> MIMDKSIPKATAKRLSLYYRIFKRFNTDGIEKASSKQIADALGIDSATVRRDFSYFGELGRRGFGYDVKKLMNFFAEILNDHSTTNVMLVGCGNIGRALLHYRFHDRNKMQISMAFDLDSNDLVGKTTEDGIPVYGISTINDHLIDSDIETAILTVPSTEAQEVADILVKAGIKGILSFSPVHLTLPKDIIVQYVDLTSELQTLLYFMNQQR

In many Gram-positive bacteria, the redox-sensing transcriptional repressor Rex controls central carbon and energy metabolism by sensing the intra cellular balance between the reduced and oxidized forms of nicotinamide adenine dinucleotide; the NADH/NAD+ ratio. Here, we report high-resolution crystal structures and characterization of a Rex ortholog (Gbs1167) in the opportunistic pathogen, Streptococcus agalactiae, also known as group B streptococcus (GBS). Rex is a homodimer consisting of two domains, an N-terminal DNA recognition domain and a C-terminal Rossmann-like dinucleotide-binding and dimerization domain. The dimerization of Rex is stabilized by the swapping of the C-terminal α-helices and the dimer binds to a consensus Rex OPerator (ROP) sequence (TTGTGAAN4TTCACAA) to repress expression of target genes.

The structure of Rex in complex with a palindromic 22 bp dsDNA fragment containing the ROP sequence (5’-AATTGTGAAATATTTCACAATT-3’, the conserved ROP consensus sequence from different bacterial species including GBS is indicated in bold) was obtained by co-crystallization and belonged to space group I222. The asymmetric unit contains a single Rex monomer bound to the corresponding half site of the ROP DNA which is predominantly in B-form, with the Rex dimer and complete ROP site related by crystal symmetry. The combined DNA-binding region of the Rex homodimer presents a striking electropositive surface that complements the bound DNA. Each Rex monomer makes a large number of phosphate and base contacts, allowing for high affinity DNA binding. The DNA-binding specificity of Rex is mediated by residues from both its wing and its helix-turn-helix regions. The wing comprises the connecting loop (residues 56–65) between helix α3 (residues 45–55) and strand β2 and packs along the side of the DNA, spanning the phosphate backbone of both strands on either side of the minor groove, involving both nonspecific contacts with the phosphate backbone, as well as specific hydrogen bond interactions between side chain of Arg62 (NH1) from the wing and N3 of adenine 3’ in the minor groove. The recognition helices (α3) of the winged helix-turn-helix motifs of the Rex dimer bind two consecutive major grooves of the ROP. Base-specific interactions involve Arg50 and Arg51 of helix α3. Specifically, nitrogen atoms (NH2) of Arg50 and Arg51 make hydrogen bonds to guanine 5 O6 and to guanine 7 O6, respectively. Ala47 makes water-mediated contacts with the bases (T6 and C16) of the major groove.> MGHHHHHHLDDLV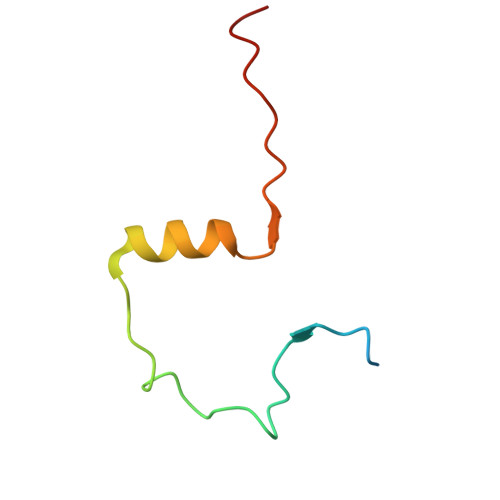AESPRKEFARINMDGIAVPDEREFDIEADMRPHELEQESDTFGAG> MFSAGHKIKGTVVLMPKNELEVNPDGSAVDNLNAFLGRSVSLQLISATKADAHGKGKVGKDTFLEGINTSLPTLGAGESAFNIHFEWDGSMGIPGAFYIKNYMQVEFFLKSLTLEAISNQGTIRFVCNSWVYNTKLYKSVRIFFANHTYVPSETPAPLVSYREEELKSLRGNGTGERKEYDRIYDYDVYNDLGNPDKSEKLARPVLGGSSTFPYPRRGRTGRGPTVTDPNTEKQGEVFYVPRDENLGHLKSKDALEIGTKSLSQIVQPAFESAFDLKSTPIEFHSFQDVHDLYEGGIKLPRDVISTIIPLPVIKELYRTDGQHILKFPQPHVVQVSQSAWMTDEEFAREMIAGVNPCVIRGLEEFPPKSNLDPAIYGDQSSKITADSLDLDGYTMDEALGSRRLFMLDYHDIFMPYVRQINQLNSAKTYATRTILFLREDGTLKPVAIELSLPHSAGDLSAAVSQVVLPAKEGVESTIWLLAKAYVIVNDSCYHQLMSHWLNTHAAMEPFVIATHRHLS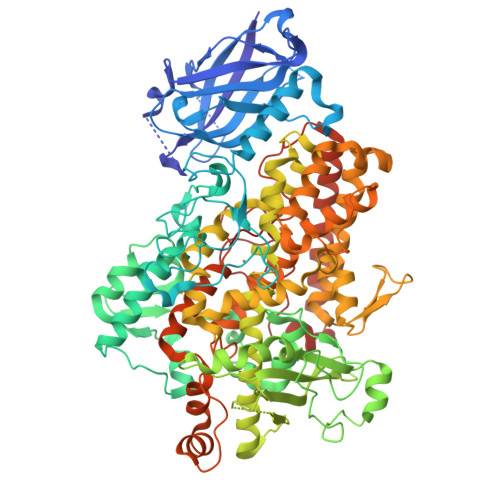VLHPIYKLLTPHYRNNMNINALARQSLINANGIIETTFLPSKYSVEMSSAVYKNWVFTDQALPADLIKRGVAIKDPSTPHGVRLLIEDYPYAADGLEIWAAIKTWVQEYVPLYYARDDDVKNDSELQHWWKEAVEKGHGDLKDKPWWPKLQTLEDLVEVCLIIIWIASALHAAVNFGQYPYGGLIMNRPTASRRLLPEKGTPEYEEMINNHEKAYLRTITSKLPTLISLSVIEILSRHASDEVYLGQRDNPHWTSDSKALQAFQKFGNKLKEIEEKLVRRNNDPSLQGNRLGPVQLPYTLLYPSSEEGLTFRGIPNSISI> MKTNPLPATPSVWGGSTVELPPTTRDTAGQGLLRRVLRPPISRRDGPGLPRGSGPRRAASTLWLLGLDGTDAPPGALTPNDDTEQALDKILRGTMRGGAALIGSPRHHLTRQVILTDLCQPNADRAGTLLLALRHPADLPHLAHQRAPPGRQTERLGEAWGQLMEATALGSGRAESGCTRAGLVSFNFLVAACAASYDARDAADAVRAHVTANYRGTRVGARLDRFSECLRAMVHTHVFPHEVMRFFGGLVSWVTQDELASVTAVCAGPQEAAHTGHPGRPRSAVILPACAFVDLDAELGLGGPGAAFLYLVFTYRQRRDQELCCVYVIKSQLPPRGLEPALERLFG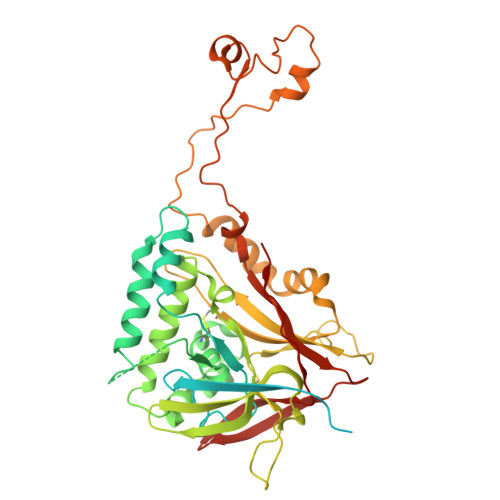RLRITNTIHGTEDMTPPAPNRNPDFPLAGLAANPQTPRCSAGQVTNPQFADRLYRWQPDLRGRPTARTCTYAAFAELGMMPEDSPRCLHRTERFGAVSVPVVILEGVVWRPGEWRACA> GQEERNQQQDDIEELETKAVGMSNDGRFLKFDIEIGRGSFKTVYKGLDTETTVEVAWCELQDRKLTKSERQRFKEEAEMLKGLQHPNIVRFYDSWESTVKGKKCIVLVTELMTSGTLKTYLKRFKVMKIKVLRSWCRQILKGLQFLHTRTPPIIHRDLKCDNIFITGPTGSVKIGDLGLATLKRASFAKAVIGTPEFMAPEMYEEKYDESVDVYAFGMCMLEMATSEYPYSECQNAAQ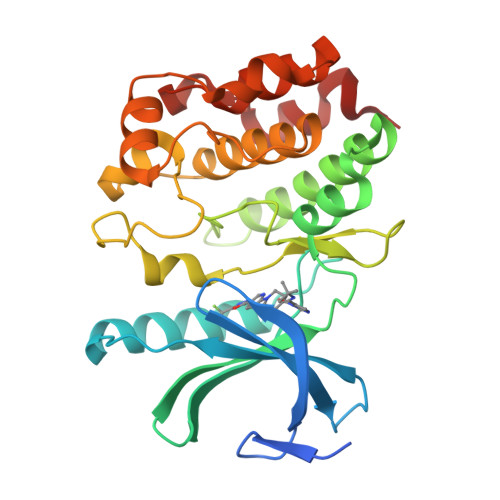IYRRVTSGVKPASFDKVAIPEVKEIIEGCIRQNKDERYSIKDLLNHAFFQEET>MAFKVISQENLLEQKRKETLQEDIPFIVNGEMEYVTKKISNGEMETLELNKPLGEMMTFSSTSNLKELLRKVVLDVELGREQVQLLYKPIYDSIADSNLPQVMDAKWALQGNCVFLEHIEGEEIKFGTINAENGPVARIQTYATGFEYTKEMKDFNQTFSVEILNKSIGESYNALLNHIHLSPIINFNYKASNKTAFKGETNDPIWLGIWRTLTQAQKDTVIAKRQGNILMASSADQIEIEMALNGGHLLNGSMYPSIKNISTVIYYDGWEVTVGKKTYSYKGVTPGKGYLIRPKRGFKELIKRDLTTEVGNADLSKLVENQIVGHCYRGAFAAVEENVQEISFR[7x];>MAFKGQPTPSTITQITRAKISDGKSVRVILSEGESTKTQQFYLINGFFGVAMQDGEKGDEVTLQIEQAEYETDNIVTSEAFEAGKLIYWDNTAKKFTTTSASNRLVGRVTDGKDSNNVIWFILLPQQ[7x]

Here, we reveal the extended and contracted atomic structures of an intact contractile-tailed phage (φCD508) that binds to and penetrates the protective S-layer of the Gram-positive human pathogen Clostridioides difficile. The virion can be divided into five distinct regions: the head, neck, tail, baseplate, and needle. Structures of purified φCD508 virions in both extended and contracted conformations were determined by single-particle EM of frozen-hydrated samples; the resolution ranged from 2.6 to 4.0 Å for the extended phage, and 2.9 to 4.2 Å for the contracted form.

The 650-Å-diameter head is formed of a near-complete T = 7 icosahedral capsid and houses the genomic DNA. It is made up of 415 and 420 copies of two capsomer proteins, the major capsid protein gp49 and the capsid decoration protein gp48, respectively. Within the capsid of the extended phage, internal density shows layers of packaged DNA.>[2x]MTINTALPTPRAPTGISVI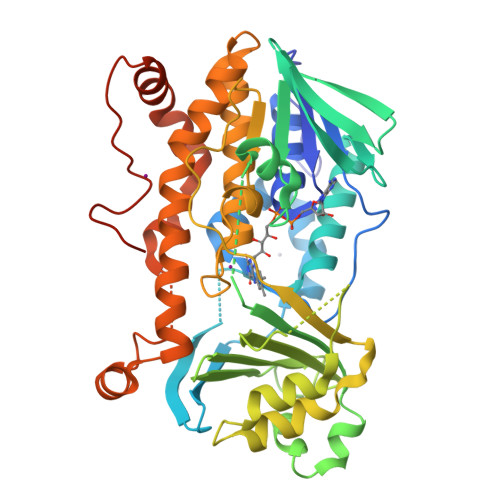VVGLGFGGLTAAIESHLRGHSVILLEKVTKVKQDAGDAIVIGPNAVRLIKSWGEQLCEEIEPHLSNATHAEMLDHHDRFIVRHELAGRGKGWFTNRGRLISILYEHARKLGIDIRLGSRVTKYWEEDGRAGVIVNDRERLAADCVICADGVHSAARAWLTGQVDTQQHSGWANFRAHMTTEQLAKDPEASWVLQGTREKDRVYVWFGDGINLAIMTMKRGQELAWALMHTDKFNAHESWAGGRASIDDALATLSPWPGRLRPSSVIRHTLPEKLVDHALIYRPPLDTWVSAGGRVMLIGDAAHPYFPVVGQGGSQAIEDGVVVATALELAGKENVPLALRVAEKIRYPRATVIQLGSSTLQEHLFWPDWEAVAKDPSVFAFPNPEWILGHDCREYTHQVFDTVVRAVRGEGEYIPRNIPADGAYRVEDTYSPEGHHHHHH>[4x]SHMDPVSVWGNTPLATVDPEIHDLIEKEKRRQCRGIELIASENFTSFAVIEALGSALTNKYSEGMPGNRYYG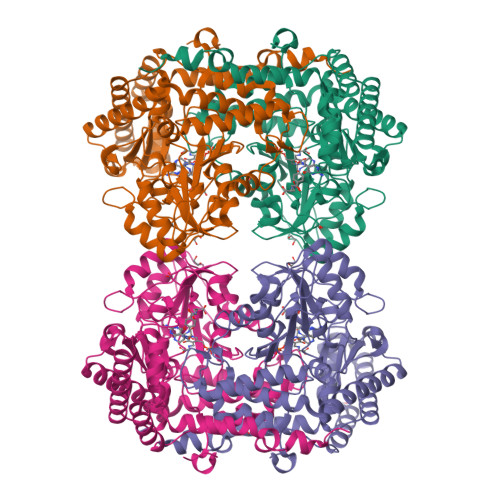GNEYIDQIENLCRSRALQAFHLDAQSWGVNVQPYSGSPANFAAYTAVLNPHDRIMGLDLPSGGHLTHGYYTSGGKKISATSIYFESLPYKVNSTTGYIDYDRLEEKALDFRPKLIICGGSAYPRDWDYKRFREVADKCGALLLCDMAHTSGLVAAQEVNSPFEYCDIVTTTTHKSLRGPRAGMIFYRKGPKPPKKGQPENAVYDFEDKINFAVFPSLQGGPHNHQIGALAVALKQAASPGFKAYAKQVKANAVALGKYLMGKGYSLVTGGTENHLVLWDLRPLGLTGNKVEKLCDLCNITVNKNAVFGDSSALAPGGVRIGAPAMTSRGLVEKDFEQIGEFLHRAVTLTLEIQKEHGKLLKDFNKGLVNNKAIEDLKADVEKFSALFDMPGFLVSEMKYKD>[60x]MAKQQNNRRKSATMRAVKRMINTHLEHKRFALINSGNTNATAGTVQNLSNGIIQGDDINQRSGDQVRIVSHKLHVRGTAITVSQTFRFIWFRDN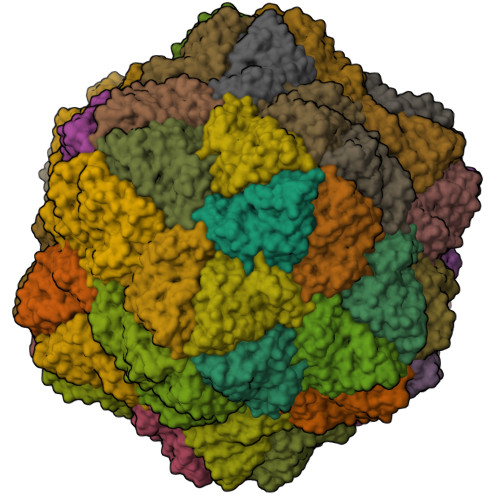MNRGTTPTVLEVLNTANFMSQYNPITLQQKRFTILKDVTLNCSLTGESIKDRIINLPGQLVNYNGATAVAASNGPGAIFMLQIGDSLVGLWDSSYEAVYTDA>[3x]MSELLVYMNGEFVPESQAKVSVFDHGFLYGDGVFEGIRAYNGKVFKLYEHIDRLYDCARVIDLKIPLSKEEFAEAILETLRRNNLRDAYIRPIVTRGAGDLGLDPRKCPSPNVIIITKPWGKLYGDLYEKGLKAITVAIRRNAIDSLPPNIKSLNYLNNILAKIEANAKGGDEAIFLDHNGYISEGSGDNIFIVKNGTITTPPTLNNLKGITRQVVIELINELEIPFREANIGLFDLYSADEIFVTGTAAEIAPVTYIDGRTVGNGKPGKVTKMLMEKFRERTENEGVEIYR

Branched chain TAms (BCATs) catalyse reversible transamination of branched chain amino acids. The subunit of the archaeal BCATs has a PLP type IV fold typical of other BCATs, D-amino acid TAms and (R)-selective ωTAms and consists of two α/β domains, a small domain and a large domain connected by two inter-domain loops. A dimer formation is required for the BCAT catalytic activity, since residues from both subunits in the dimer contribute to the active site.

The GEO1900 holoform (internal aldimine form; GEO1900_holo) and the unproductive complex of holoenzyme with the keto substrate AKG-(GEO1900_AKG) have been determined to 1.9 and 2.2 Å resolution, respectively, in the trigonal space group P3221. There are three GEO1900 subunits per asymmetric unit, which form a tight hexamer with 32 point group symmetry with their symmetry mates. A PLP molecule is covalently bound to the catalytic Lys152 in the GEO1900 active site (Lys150 in AF0933). Apart from the Schiff base formed by the NZ of Lys152 residue, the pyridine ring of the cofactor forms hydrogen bonds to the conserved Tyr156 and Glu185 residues. The PLP phosphate group forms a salt bridge with Arg53 and a number of hydrogen bonds to the main chain nitrogens and side chains of residues Thr212 and Thr248, and the main chain nitrogen of Ile211, and two water molecules. In the GEO1900_holo structure the inter-domain loop is not seen in the electron density for subunits A and C, but in subunit B only two residues 120–121 are not observed. The other residues of the inter-domain loop have higher B factors than the average B factor of the model. In the case of the GEO1900_holo structure the conformations of the flexible loops have small differences between the different subunits. However, these are likely to be due to crystal packing effects. When purified by high resolution gel filtration chromatography the native molecular weight of the two enzymes varied with the GEO1900 approximately 70 kDa, indicating that the enzyme was a homodimer with small amount of tetramer in solution.> MS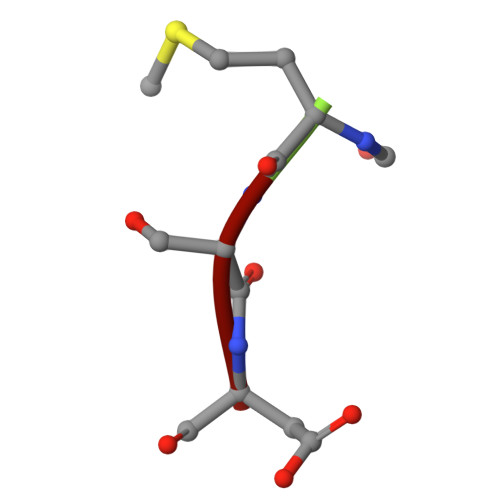D> DPNRAPPCDSSQCVLPDCFCSEDGTVIPGDLPARDVPQMITITFDDAINNNNIELYKEIFNGKRKNPNGCDIKATYFVSHKYTNYSAVQETHRKGHEIAVHSITHNDDERFWSNATVDDWGKEMAGMRVIIEKFSNITDNSVVGVRAPYLRVGGNNQFTMMEEQAFLYDSTITAPLSNPPLWPYTMYFRMPHRCHGNLQSCPTRSHAVWEMVMNELDRREDPSNDEYLPGCAMVDSCSNILTGDQFYNFLNHNFDRHYEQNRAPLGLYFHAAWLKNNPEFLEAFLYWIDEILQSHNDVYFVTMTQVIQWVQNPRTVTEAKNFEPWREKCSVEGNPACWVPHSCKLTSKEVPGETINLQTCLRCPVNYPWLNDPTGDGHYHHHHHH

Carbohydrate esterase 4 family (CE4)2 chitin deacetylases (CDAs, EC 3.5.1.41) catalyze the removal of acetyl groups from chitin to form chitosan, a polymer of β-(1,4)-linked d-glucosamine residues. CDAs are widely distributed in protists, diatoms, bacteria, fungi, nematodes, and insects, playing vital roles in chitinous matrix formation and modification, as well as in biological attack of fungal pathogens. In this study, two CDAs from Bombyx mori, BmCDA1 and BmCDA8, were crystallized and resolved, providing the first insight into the structural characteristics, activity profiles, and deacetylation mode of insect CDAs. The structures revealed that insect CDAs possess several unique structural features that distinguish them from other known CE4 enzymes.

BmCDA1 is composed of an N-terminal signal region (residues 1–23), a chitin-binding domain (residues 24–122), a low-density lipoprotein receptor domain (residues 123–161), and a catalytic domain (CAD, residues 162–539). Our experiments showed that full-length recombinant BmCDA1 was not stable and underwent autocleavage when incubated with the crystallization reagent. Thus, the truncated form of BmCDA1 (BmCDA1-CAD, residues 162–539) was cloned, expressed, and purified for crystallization. Diffraction data were collected to 1.98 and 2.4 Å on native and SeMet protein crystals, respectively, and the structure was solved using the SeMet single-wavelength anomalous diffraction technique. The overall structure of BmCDA1-CAD consists of two regions: a CE4-conserved NodB homology subdomain and C-terminal loops. The active site of BmCDA1-CAD is located at the top center of the (β/α)7 barrel and contains a metal-binding triad conserved across the CE4 family, namely, a zinc ion coordinated by Asp206, His261, and His265. Taken together, the differences in motif 4 and motif 5 confer BmCDA1 a more open and wider active pocket. The substrate-binding cleft is shallow and open when compared with the other microbial CDAs because of the lack of several loops that give microbial CDAs their characteristically deep and narrow substrate-binding cleft. Our study showed that the deacetylation activity of BmCDA1 was undetectable toward various chitinous substrates even with prolonged incubation time to 120 h or with higher enzyme concentrations at 200 μm. Taken together, these data indicated that BmCDA1 requires specific accessary proteins to achieve activity.4-(isoquinolin-3-ylamino)-4-oxobutanoic acid | C13 H12 N2 O3 | 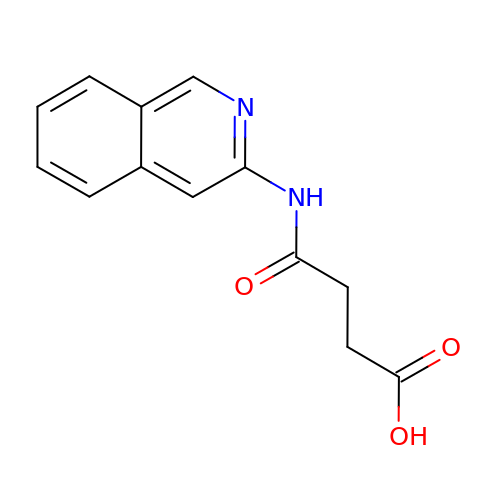CJIVLGFQCOFDOG-UHFFFAOYSA-N> MVMKASVDDDDSGWELSMPEKMEKSNTNWVDITQDFEEACRELKLGELLHDKLFGLFEAMSAIEMMDPKMDAGMIGNQVNRKVLNFEQAIKDGTIKIKDLTLPELIGIMDTCFCCLITWLEGHSLAQTVFTCLYIHNPDFIEDPAMKAFALGILKICDIAREKVNKAAVFEEEDFQSMTYGFKMANSVTDLRVTGMLKDVEDDMQRRVKSTRSRQGEERDPEVELEHQQCLAVFSRVKFTRVLLTVLIAFTKKETSAVAEAQKLMVQAADLLSAIHNSLHHGIQAQNDTTKGDHPIMMGFEPLVNQRLLPPTFPRYAKIIKREEMVNYFARLIDRIKTVCEVVNLTNLHCILDFFCEFSEQSPCVLSRSLLQTTFLVDNKKVFGTHLMQDMVKDALRSFVSPPVLSP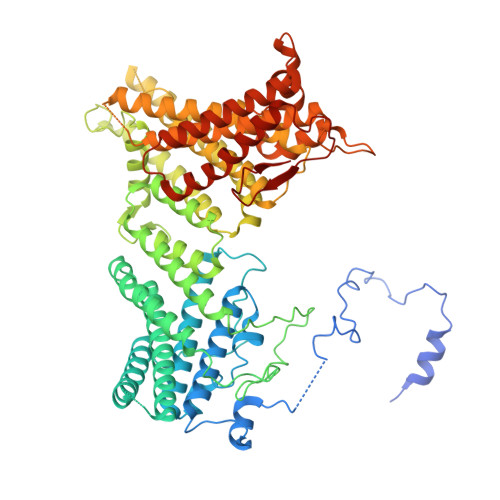KCYLYNNHQAKDCIDSFVTHCVRPFCSLIQIHGHNRARQRDKLGHILEEFATLQDEAEKVDAALHTMLLKQEPQRQHLACLGTWVLYHNLRIMIQYLLSGFELELYSMHEYYYIYWYLSEFLYAWLMSTLSRADGSQMAEERIMEEQQKGRSSKKTKKKKKVRPLSREITMSQAYQNMCAGMFKTMVAFDMDGKVRKPKFELDSEQVRYEHRFAPFNSVMTPPPVHYLQFKEMSDLNKYSPPPQSPELYVAASKHFQQAKMILENIPNPDHEVNRILKVAKPNFVVMKLLAGGHKKESKVPPEFDFSAHKYFPVVKLV> MSAKPTTVVLYPSPGMGHLVSMFELAKLLDRHGLSVTVIIVEPHYNTGSTAAFIARSSASNPSVSFRVLPRPDSLPHNPSRHHEAHAFDLLRLSNPELRRFLLESPPSALVLDYFCGNALDVSAELRIPAYYFFTSGAGVLSAFLHFPDLHSRTAASFREMGSSPLHFPGIPPLPADHMPVPMLDRDDPVYESFLYFSKRLKEAEGYIINTFEDLEPRAVAAISDAALPPNYCIGPLIQSRDRESSSSRGGSECLAWLDAQPKRSVVFLCFGSIGLFSSEQLKEMAVGLERSGQRFLWVVRSPPSGDSDKLFEAPREPDLERILPEGFLERTEGRGLVVKSWAPQAAVLEHGSVGGFVTHCGW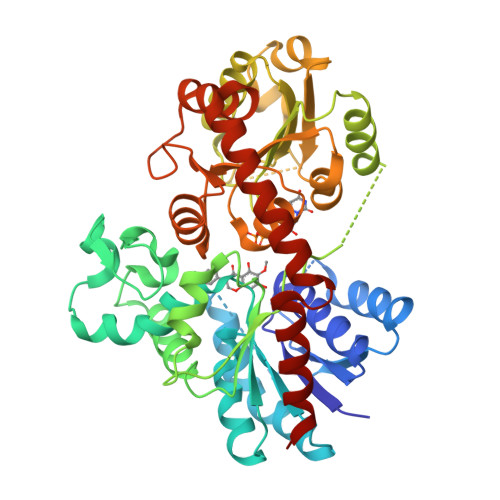NSTLEAIASGVPMVAWPMYAEQWMNKVFLVEEMKLAVPMEGYDKDMVTAEEVERKVRWLMESEGGVELRARTERAKERAAASLAEGGKSKVALLEVVERMKRGI>SNAMRHDEYQYLDLIRQIMRTGNRKGDRTGTGTISMFGAQMRYSLRDGIFPLLTTKRVFWRGVAEELLWFVRGSTNAKELQEKDIHIWDGNSSKEFLNKMGFHDREEGDLGPVYGFQWRHFGAPYADMHTDYTGQGVDQ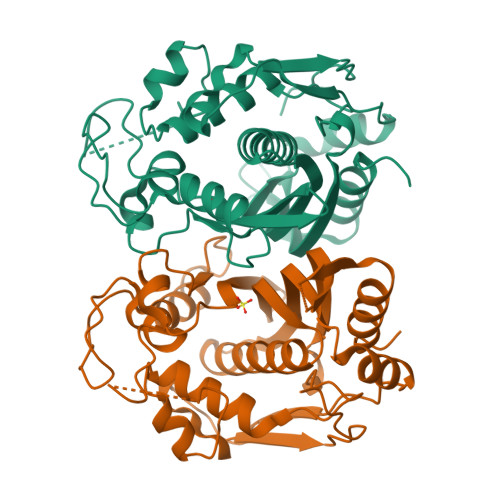LQQVIDTIKNNPDDRRIIMCAWNPVDVPKMALPPCHCLCQFYVANGELSCQLYQRSADMGLGVPFNIASYALLTYMIAHVTDLKPGDFVHTLGDAHVYSNHCEALEEQLKREPRPFPSLKIKRKVENISDFKFEDFELDGYKPHPKIKMEMAV[16x]2-methyl-~{N}-[(2~{R})-1-methylsulfonylpropan-2-yl]pyridin-3-amine | C10 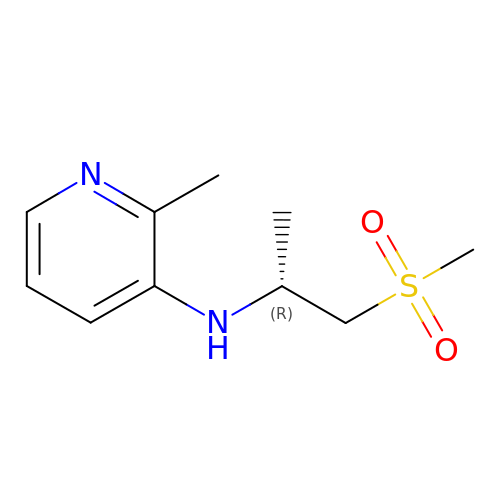H16 N2 O2 S | HXYSCWJADZACTE-MRVPVSSYSA-N>MVKAAAAAASAPTGPGIYSATYSGIPVYEYQFGLKEHVMRRRVDDWINATHILKAAGFDKPARTRILEREVQKDQHEKVQGGYGKYQGTWIPLEAGEALAHRNNIFDRLRPIFEFSPGPDSPPPAPRHTSKPKQPK[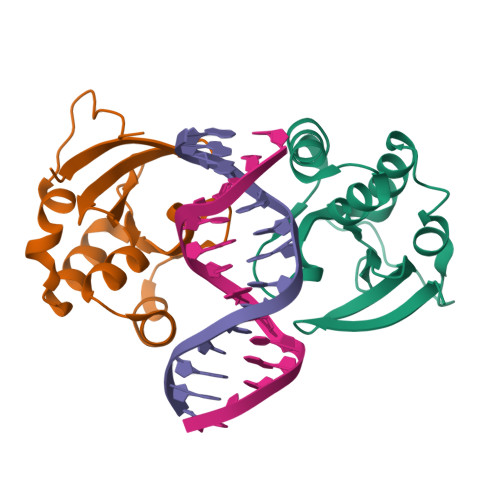2x]> GAMKKVEILMVVDAAAALASRDLQSNIYLIDTNKYMGSGNEGQAELKTACKDGQLLCWRVVAISPDNEVDIVEFNGQMINDRVCIPTKQGLSGDEFWEGRVEAQGQASTQQYNATLSIDGSRLTFDPFLVISL

While the cholera toxin is the primary virulence factor, V. cholerae also expresses other virulence factors, such as the tripartite toxin MakABE that is secreted via the bacterial flagellum. MakABE are co-expressed with two accessory proteins, MakD and MakC, which are encoded by the same makDCBAE operon, although their functions remain unknown. Here, we present the crystal structures of MakC and MakD, revealing that they are similar in both sequence and structure but lack other close structural relatives. The structures are very similar with a root mean square deviation (RMSD) of 0.45 Å calculated on 126 Cα-atoms. Both feature a central β-sandwich, one sheet comprising six β-strands, and one with four β-strands.

To determine the crystal structure of MakC, a construct encoding the full length MakC, with an N-terminal cleavable histidine tag, was designed and expressed in E. coli. Consequently, SeMet labeled MakC was prepared, yielding needle-like crystals. The crystals, which belonged to space group C2221 and contained one molecule in the asymmetric unit, diffracted to 2.0 Å. The structure of MakC was determined by SAD phasing on SeMet labeled protein. In MakD, two dimers were present in the asymmetric unit, whereas the MakC dimer is formed by crystallographic symmetry. Both the MakC and MakD homodimers are formed by the interaction between identical surfaces in each subunit, head-to-tail, (β5123 pack anti-parallel to the equivalent strands, β5’1′2′3′ of the other subunit). As calculated by PISA, each MakC subunit buries approximately 1,050 Å2 and each subunit of MakD 943 Å2. In MakC, the residue in the equivalent position is a valine, and there are no other cysteines in MakC that could potentially form disulfide bonds in the dimer-dimer interface. The equivalent β-sheet of MakC is less hydrophobic based on the electrostatic potential map, and the polar residues are more evenly distributed. On the contrary, analysis with MakC antisera revealed that MakC forms large complexes within the bacterial cell, as evidenced by a reduction in the amount of monomeric protein following treatment, which varied with both time and glutaraldehyde concentration.>MRKKISIIGAGFVGSTTAHWLAAKELGDIVLLDIVEGVPQGKALDLYEASPIEGFDVRVTGTNNYADTANSDVIVVTSGAPRKPGMSREDLIKVNADITRACISQAAPLSPNAVIIMVNNPLDAMTYLAAEVSGFPKERVIGQAGVLDAARYRTFIAMEAGVSVQDVQAMLMGGHGDEMVPLPRFSTISGIPVSEFIAPDRLAQIVERTRKGGGEIVNLLKTGSAYYAPAAATAQMVEAVLKDKKRVMPVAAYLTGQYGLNDIYFGVPVILGAGGVEKILELPLNEEE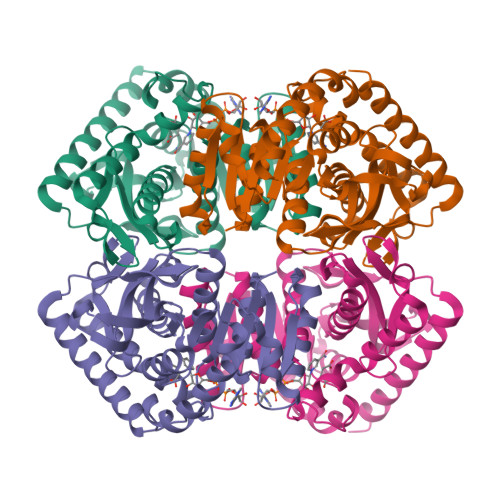MALLNASAKAVRATLDTLKSL[2x]> GMVRYPLEPV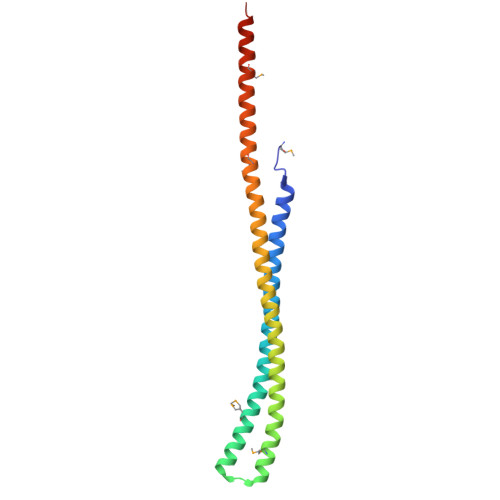LSIKKDRVDRAEKVVKEKRRLLELEQEKLRERESERDKVKNHYMQKIRQLREQLDDGTTSDAILKMKAYIKVVAIQLSEEEEKVNKQKENVLAASKELERAEVELTKRRKEEEKTRLHKEEWMKEALKEEARQEEKEQDEMGQLLHQLHKQKQRESGEN>MDKLISNNKLKLSVVL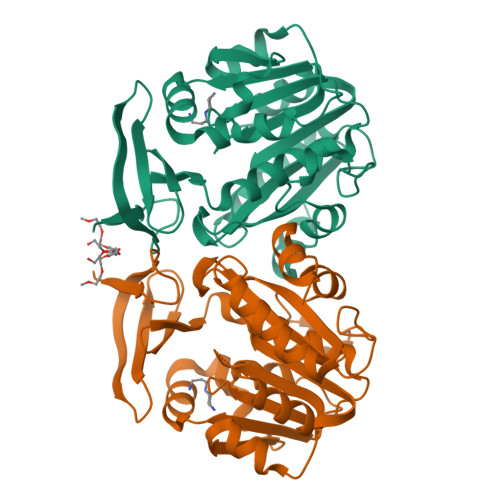LGGLCSLAYYHLKNKFHLSQFCFSKKWFSEFSIMWPGQAFSLKIKKILYETKSKYQNVLVFESTTYGKVLVLDGVIQLTEKDEFAYHEMMTHVPMTVSKEPKNVLVVGGGDGGIIRELCKYKSVENIDICEIDETVIEVSKIYFKNISCGYEDKRVNVFIEDASKFLENVTNTYDVIIVDSSDPIGPAETLFNQNFYEKIYNALKPNGYCVAQCESLWIHVGTIKNMIGYAKKLFKKVEYANISIPTYPCGCIGILCCSKTDTGLTKPNKKLESKEFADLKYYNYENHSAAFKLPAFLLKEIENI[3x]> MASSYSASAEPARVRALVYGHHGDPAKVVELKNLELAAVRGSDVRVKMLAAPINPSDINMIQGNYGLLPELPAVGGNEGVAQVVAVGSNVTGLKPGDWVIPANAGLGTWRTEAVFSEEALIQVPSDIPLQSAATLQVNPCTAYRMLMDFEQLQPGDSVIQNASNSGVGQAVIQIAAALGLRTINVVRDRPDIQKLSDRLKSLGAEHVITEEELRRPEMKNFFKDMPQPRLALNCVGGKSSTELLRQLARGGTMVTYGGMAKQPVVASVSLLIFKDLKLRGFWLSQWKKDHSPDQFKELILTLCDLIRRGQLTAPACSQVPLQDYQSALEASMKPFISSKQILTMLEHHHHHH

Mitochondrial fatty acid synthesis (mtFAS) is essential for respiratory function. The last step of mtFAS is carried out by 2E-enoyl-ACP thioester reductases MECR and Etr1 in human and yeast, respectively. These enzymes are members of the medium-chain dehydrogenase / reductase (MDR) superfamily, catalyzing the NADPH-dependent reduction of 2E-enoyl thioesters into acyl thioesters. The structure of MECR shows a bent cavity of sufficient dimensions to accommodate acyl substrates with carbon chain lengths from C4 to C1619.

Our in vitro and in vivo analyses indicate that the MECR G165Q variant allows synthesis of octanoyl groups but not long chain fatty acids, confirming the validity of our computational approach to engineer substrate length specificity. The electron density map of the MECR G165Q crystal structure shows the structural changes due to the mutation. The structure of the Q165 side chain is well defined by the electron density map. The mutation site locates in the domain interface in between the α helix αD of the catalytic domain and α helix αA of the cofactor binding domain. The side chain points across the acyl tail binding tunnel, making a good hydrogen bond between NE2(Q165) and O(P130). This interaction causes changes in the main chain conformation of the residues near P130 and Q165, as well as of the side chain conformations of K316 and E107. Furthermore, in wild-type MECR, the side chain of K316 is hydrogen bonded to the backbone oxygen of G165, but in the MECR G165Q variant, the lysine side chain is hydrogen bonded with the side chain of Q165 and the backbone oxygen of P130. The introduction of the glutamine side chain to the position 165 neither affected the overall structure, nor the conformation of the catalytic tyrosine (Y94) or the NADPH binding site, but together with conformational changes of an acidic (E107) and basic (K316) amino acid, the modification induces a change of the acyl binding cavity of the mutated protein. As a result, the fatty acyl binding cavity is much shorter in the MECR G165Q variant. Clearly, the G165Q mutation blocks the acyl tail binding tunnel, in good agreement with the changed substrate specificity.> MTSVTRSEIIDEKGPVMSKTHDHQLESSLSPVEVFAKTSASLEMNQGVSEERIHLGSSPKKGGNCDLSHQERLQSKSLHLSPQEQSASYQDRRQSWRRASMKETNRRKSLHPIHQGITELSRSISVDLAESKRLGCLLLSSFQFSIQKLEPFLRDTKGFSLESFRAKASSLSEELKHFADGLETDGTLQKCFEDSNGKASDFSLEASVAEMKEYITKFSLERQTWDQLLLHYQQEAKEILSRGSTEAKITEVKVEPMTYLGSSQNEVLNTKPDYQKILQNQSKVFDCMELVMDELQGSVKQLQAFMDESTQCFQKVSVQLGKRSMQQL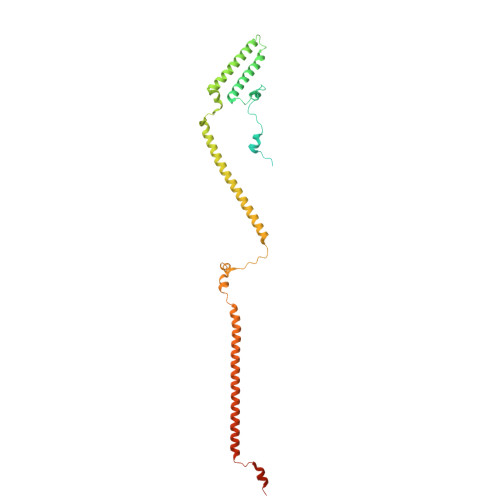DPSPARKLLKLQLQNPPAIHGSGSGSCQ>[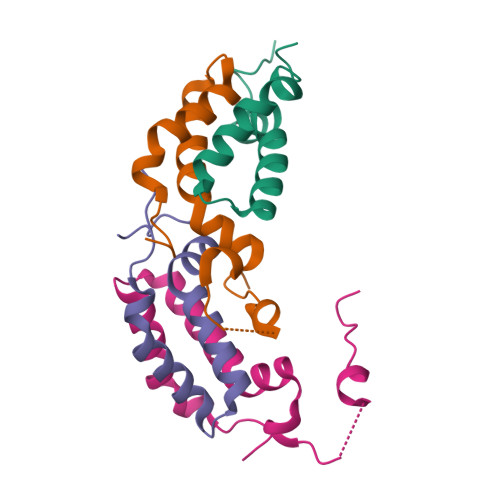2x]MEPEQMLEGQTQVAENPHSEYGLTDNVERIVENEKINAEKSSKQKVDLQSLPTRAYLDQTVVPILLQGLAVLAKERPPNPIEFLASYLLKNKAQFEDRNLERPHRD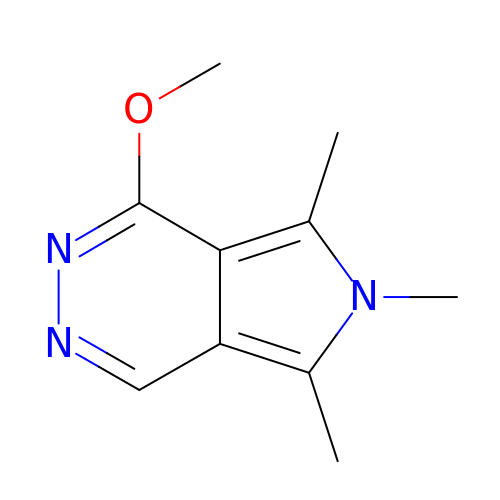4-methoxy-5,6,7-trimethyl-pyrrolo[3,4-d]pyridazine | C10 H13 N3 O | JBVFAOAKSYCBHG-UHFFFAOYSA-N>[8x]MSKIAPQCQNLREQVNQLIELLRQEPTLRSQQDTSIVETALGKALSPRFEIVFAGAFSAGKSMLINALLERELLYSAEGHATGTECHIEYANANEERVVLTFLSEAEIRQQALILAKYLNVNVGDLNINQPEAVKVVSQYCQKIIAEEGGENKSERAKQANALHLLLIGFEQNRERINTVQNSTYSMDQLNFSSLAEAAGYARRGANSAVLKRLDYFCNHSLLKDGNVLVDLPGIDAPVKEDAERAYRKIESPDTSAVICVLKPAAAGDMSAEETQLLERISKNHGIRDRVFYVFNRIDDTWYNTQLRQRLEGLIQSQFRDNSRVYKTSGLLGFYGSQVKQTNSSTRFGLDSIFATTIKGFDGEEETPQFVSEFNNYCANSGKLLSTAFRVSVNGYETSNENYVRILSEWGIPLVDQLIHDSGIESFRSGIGLYLAEEKYPELFATLANDLQPLCIALRQFYLENYRQLDSQPREIAAMKAQELTLLNQEMQNLGIEFKKYMSAQINDVVIGNDREFDQDFTKLKARMVARLDELLKTFSVMNAYKRATESHPRNSTAPFIAVLVEALYYLANELEDAFIEAIHELVKNFFQRLGDRLRKVDCYHQVYRLVGNDGGIEQLLRRAEEDITKALVNEARTECDRYVRESPRFYDEGTFSIYQFRQTLQQTSQGYDAQAIVEAEPAIKELLKLDFEPKVFNTVRKNFRQTVNNTLKTHLLPMAEEQAQIILEQYDVARKYREQTLEQDAEEKIARNSRLQSEIKQKIDLYQTSIVSINECLKAMQIFEQLPVITESDITKQAEIVADADFVEIVELEHHHHHH

Unlike small (Ras-like) GTPases, DLPs are large mechanochemical GTPases with a molecular mass >60 kDa that use the energy gained via GTP hydrolysis for membrane binding and/or remodeling. While DLP family members are typically not highly conserved on the sequence level, with the exception of the GTPase domain (GD), the resolved structures reveal a conserved modular arrangement of all DLPs: The globular GD at the protein’s N-terminus is typically followed by an α-helical bundle signaling element (BSE) or neck domain that connects the GD to an α-helical stalk or trunk domain. Recently, a BDLP has also been identified in the genome of the cyanobacterium Synechocystis sp. PCC 6803 (SynDLP). Taken together, the recently predicted cyanobacterial DLP of Synechocystis sp. PCC 6803 (SynDLP) is a bona fide member of the dynamin superfamily as classified by activity and structure.

Yet, in contrast to other BDLPs, SynDLP forms high-molecular mass oligomers already in complete absence of an externally added membrane template and/or nucleotides. Using a segmented single-particle analysis workflow, we determined the structure of SynDLP oligomers at an overall resolution of 3.7 Å. Based on the determined cryo-EM map, we built a model of 8 SynDLP monomers, which represents a smaller part of the segmented SynDLP oligomer structure. The last 19 residues at the C-terminus could not be resolved in the cryo-EM density, and thus, the final refined atomic model includes amino acids (aa) 1-793 of SynDLP. The monomer model revealed a globular GD, linked via a flexible hinge region (hinge 2) to the mainly α-helical BSE domain, which is connected to an α-helical stalk via hinge 1. The oligomer structure showed a stalk backbone connected via a complex interaction network from which the BSE domains and the GDs protrude laterally outwards. The structure of SynDLP oligomers resembles the assembly of eukaryotic fission DLPs via a complex network of interactions in the stalk domain, mainly mediated by three distinct interfaces. The SynDLP structure indicated the formation of an intramolecular disulfide bridge between C8 and C777 that covalently connects the BSE1 and BSE3 domains. The structure of the SynDLP oligomers revealed only a small interface between adjacent GDs, whereas a large area of the GD of monomer 1 contacts the BSE1 domain of monomer 2. Yet, the determined cryo-EM structure of SynDLP did not indicate transverse contacts between GDs of adjacent monomers.>[2x]MVQPAAWQVASLADRYEESFDIGAAVEPHQLNGRQGKVLKHHYNSIVAENAMKPISLQPEEGVFTWDGADAIVEFARKNNMNLRFHTLVWHNQVPDWFFLDEEGNPMVEETNEAKRQANKELLLERLETHIKTVVERYKDDVTAWDVVNEVVDDGTPNERGLRESVWYQITGDEYIRVAFETARKYAGEDAKLFINDYNTEVTPKRDHLYNLVQ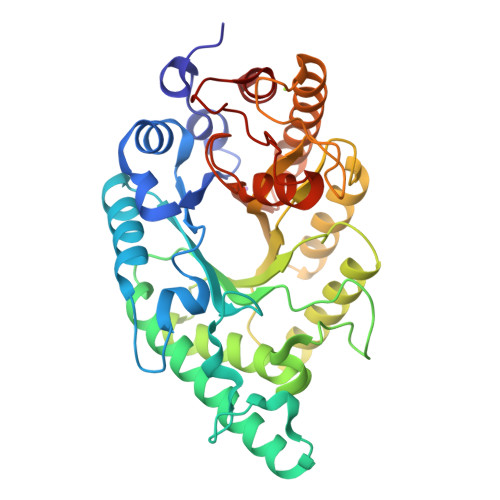DLLADGVPIDGVGHQAHIQIDWPTIDEIRTSMEMFAGLGLDNQVTELDVSLYGWPPRPAFPTYDAIPQERFQAQADRYNQLFELYEELDADLSSVTFWGIADNHTWLDDRAREYNDGVGKDAPFVFDPNYRVKPAFWRIID> GDRVADVIESSIGDSVSRALTHALPAPTGQNTQVSSHRLDTGKVPALQAAEIGASSNASDESMIETRCVLNSHSTAETTLDSFFSRAGLVGEIDLPLEGTTNPNGYANWDIDITGYAQMRRKVELFTYMRFDAEFTFVACTPTGEVVPQLLQYMFVPPGAPKPDSRESLAWQTATNPSVFVKLSDPPAQVS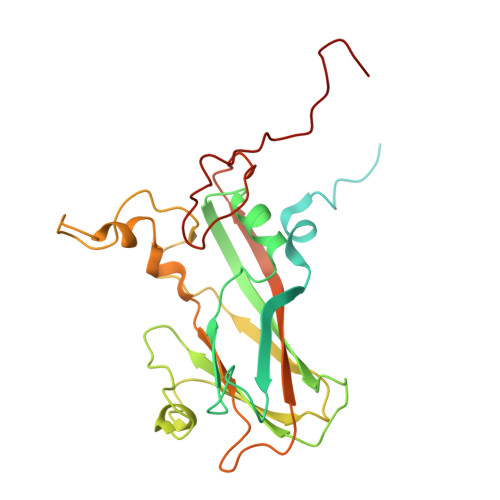VPFMSPASAYQWFYDGYPTFGEHKQEKDLEYGACPNNMMGTFSVRTVGTSKSKYPLVVRIYMRMKHVRAWIPRPMRNQNYLFKANPNYAGNSIKPTGASRTAITTL> MASFGSRMEESIRKTVTENTVVIYSKTWCSYCTEVKTLFKRLGVQPLVVELDQLGPQGPQLQ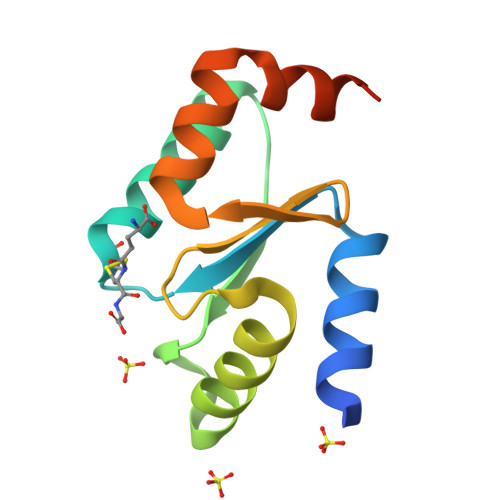KVLERLTGQHTVPNVFVCGKHIGGCTDTVKLNRKGDLELMLAEANGKNGQS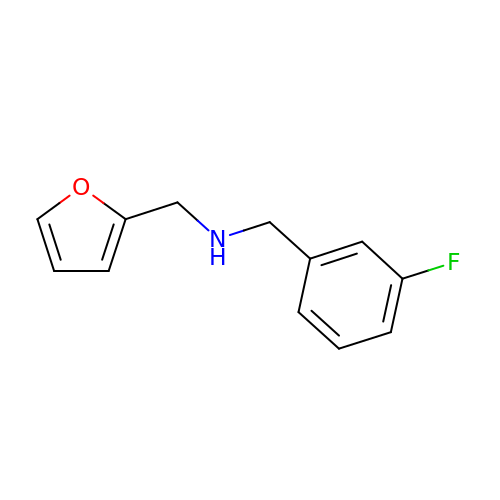1-(3-fluorophenyl)-N-[(furan-2-yl)methyl]methanamine | C12 H12 F N O | AFHNQIFVWMDQAM-UHFFFAOYSA-N8-(4-chlorophenyl)-2-phenyl-imidazo[1,2-a]pyridine | C19 H13 Cl N2 | 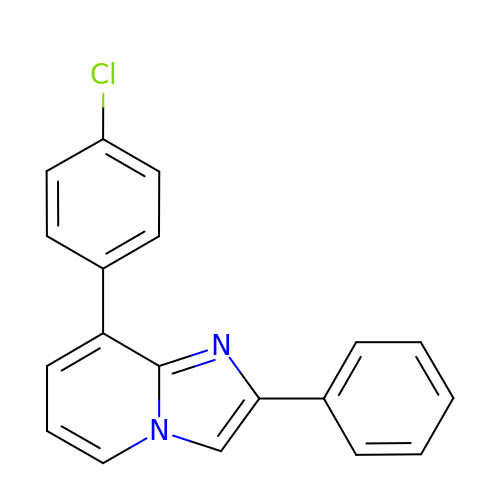PWFFYDSSTMPMCL-UHFFFAOYSA-N{2-[2-(6-oxo-1,6-dihydro-9H-purin-9-yl)ethoxy]ethyl}phosphonic 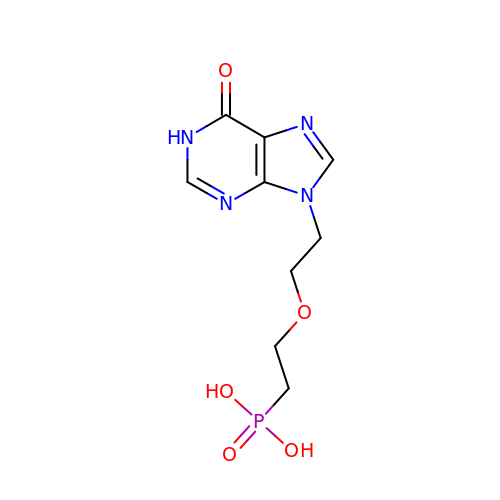acid | C9 H13 N4 O5 P | ARUATFPHVPUVFJ-UHFFFAOYSA-N> MSGHHHHHHGSEQLYFQGAMNDSILLGLIGQGLDLSRTPAMHEAEGLAQGRATVYRRIDTLGSRASGQDLKTLLDAALYLGFNGLNITHPYKQAVLPLLDEVSEQATQL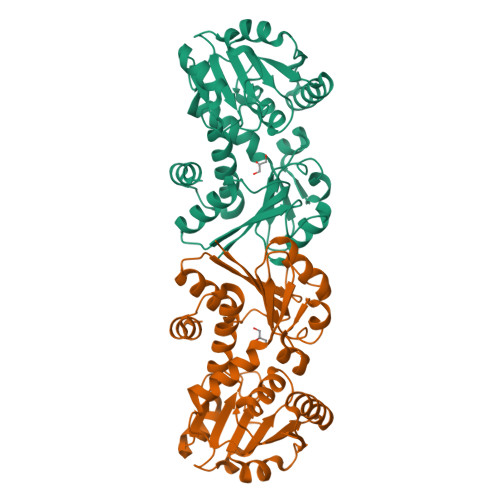GAVNTVVIDATGHTTGHNTDVSGFGRGMEEGLPNAKLDSVVQVGAGGVGNAVAYALVTHGVQKLQVADLDTSRAQALADVINNAVGREAVVGVDARGIEDVIAAADGVVNATPMGMPAHPGTAFDVSCLTKDHWVGDVVYMPIETELLKAARALGCETLDGTRMAIHQAVDAFRLFTGLEPDVSRMRETFLSL>[2x]KNSLLEKRPEDVVIVAANRSAIGKGFKGAFKDVNTDYLLYNFLNEFIGRFPEPLRADLNLIEEVACGNVLNVGAGATEHRAACLASGIPYSTPFVALNRQCSSGLTAVNDIANKIKVGQIDIGLALGVESMT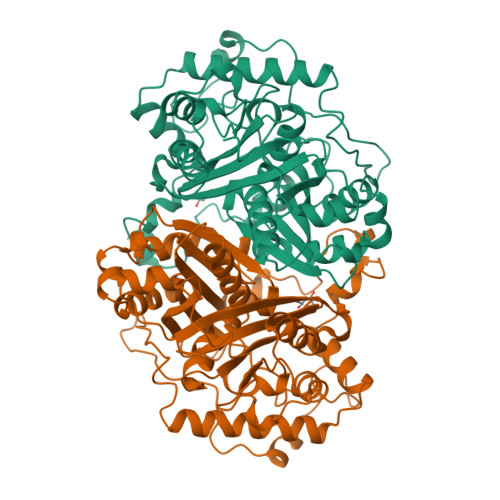NNYKNVNPLGMISSEELQKNREAKKCLIPMGITNENVAANFKISRKDQDEFAANSYQKAYKAKNEGLFEDEILPIKLPDGSICQSDEGPRPNVTAESLSSIRPAFIKDRGTTTAGNASQVSDGVAGVLLARRSVANQLNLPVLGRYIDFQTVGVPPEIMGVGPAYAIPKVLEATGLQVQDIDIFEINEAFAAQALYCIHKLGIDLNKVNPRGGAIALGHPLGCTGARQVATILRELKKDQIGVVSMCIGTGMGAAAIFIKE> SMIDDDGYRPNVGIVICNRQGQVMWARRFGQHSWQFPQGGINPGESAEQAM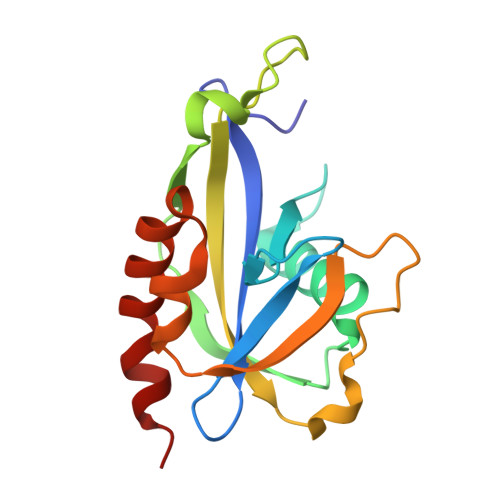YRELFEEVGLSRKDVRILASTRNWLRYKLPKRLVRWDTKPVCIGQKQKWFLLQLVSGDAEINMQTSSTPEFDGWRWVSYWYPVRQVVSFKRDVYRRVMKEFASVVMSLQ> MYLMNTYSRFPATFVYGKGSWIYDEKGNAYLDFTSGIAVNVLGHSHPRLVEAIKDQAEKLIHCSNLFWNRPQMELAELLSKNTFGGKVFFANTGTEANEAAIKIARKYGKKKSEKKYRILSAHNSFHGRTLGSLTATGQPKYQKPFEPLVPGFEYFEFNNVEDLRRKMSEDVCAVFLEPIQGESGIVPATKEFLEEARKLCDEYDALLVFDEVQCGMGRTGKLFAYQKYGVVPDVLTTAKGLGGGVPIGAVIVNERANVLEP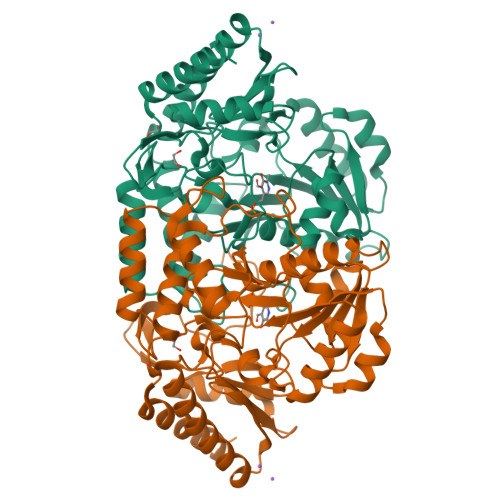GDHGTTFGGNPLACRAGVTVIKELTKEGFLEEVEEKGNYLMKKLQEMKEEYDVVADVRGMGLMIGIQFREEVSNREVATKCFENKLLVVPAGNNTIRFLPPLTVEYGEIDLAVETLKKVLQGI>GAAGAUUGUAAACAUGCCGAAAGGCAGACACUUCC[2x]

Recently, a fluorophore named 5-((Z)-4-((2-hydroxyethyl)(methyl)amino)benzylidene)-3-methyl-2-((E)-styryl)-3,5-dihydro-4H-imidazol-4-one (NBSI), emitting in red spectrum, and its cognate aptamer named Clivia were identified, exhibiting a large Stokes shift. The overall structure uses a monomeric, non-G-quadruplex compact coaxial architecture, with NBSI sandwiched at the core junction. The overall structure of the complex adopts a coaxial long helix fold and is stabilized by continuous stacking interactions from the bottom stem P1 to the apical stem P2 with the ligand NBSI intercalated in the zipped junction region at the interface of stems P1 and P2. Our structural investigation of the Clivia aptamer bound to NBSI or NBSI derivatives revealed that the Clivia aptamer adopts a non-G-quadruplex scaffold supporting a specific ligand-binding pocket, suggesting a new fluorescence activation mechanism.

To facilitate the crystallization of the Clivia complex bound to NBSI, the variable apical loop L2 of stem P2 was replaced with the stable tetraloop or protein-binding loop (cocrystallization with the RNA-binding protein), in which the GAAA tetraloop replacement generated crystals with high diffraction quality. The structure of the Clivia–NBSI complex was refined at a resolution of 1.6 Å with Rwork/Rfree values of 0.19/0.22. Each asymmetric unit contains two molecules of the Clivia–NBSI complex and minor molecular interactions were found between them. The NBSI-binding pocket is located in the central junction of the overall structure between stems P1 and P2. NBSI is sandwiched between the upper two contacting bases A15·G28 and the lower base triple U8·A29·C30, anchored by the sugar–phosphate RNA backbone between G28 and A29 and capped by two adjacently stacked residues C14 and G9. The major aromatic moieties of NBSI intercalate into the binding pocket, while the terminal (2-hydroxyethyl)(methyl)amino group of NBSI points outward from the binding pocket. Even though no direct hydrogen-bonding interaction was identified between NBSI and the Clivia aptamer in the binding pocket, water molecule W1 was found to coordinate with the N1 atom of the imidazole moiety of NBSI and form extra hydrogen bonds with the neighboring residues, potentially facilitating the specific recognition of NBSI by the Clivia aptamer. The 2-NH2 group of G28 forms a hydrogen bond with the N7 atom of A15 and a hydrogen bond with the nonbridging phosphate oxygen between A15 and C14 above the bound NBSI. The Hoogsteen edge of A29 forms a pairing interaction with the Watson–Crick edge of U8 and the N3 atom in the sugar edge of A29 forms another hydrogen bond with the 4-NH2 group of C30 below the bound NBSI.N-((2R,4S)-2-butyl-5-methyl-4-(3-(5-methylpyridin-2-yl)ureido)-3-oxohexyl)-N-hydroxyformamide | C19 H30 N4 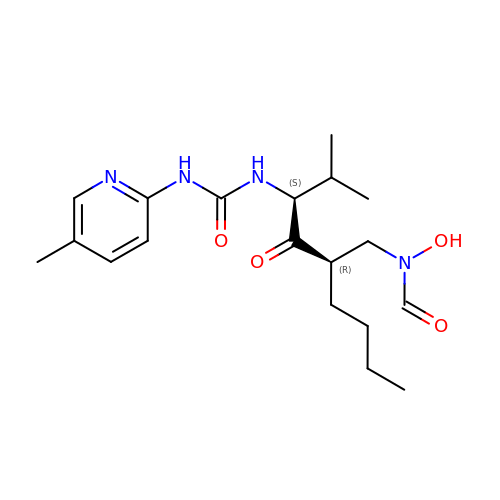O4 | AMPUUHFRILVRDV-WBVHZDCISA-N> GSSTPLVDFLMQLEDYTPTIPDAVTGYYLNRAGFEASDPRIIRLISLAAQKFISDIANDALQHCKMKGT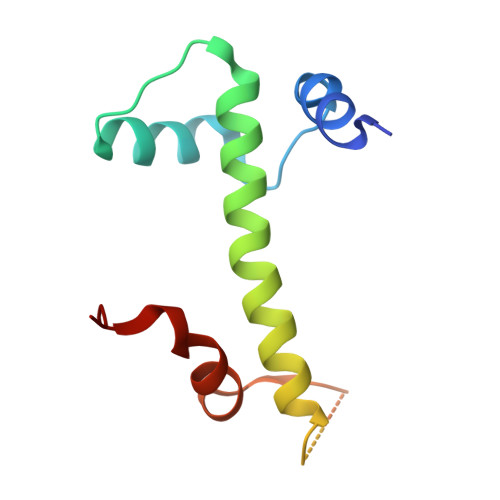ASGSSRSKSKDRKYTLTMEDLTPALSEYGINVK[[(2~{R},3~{S},4~{R},5~{R})-5-(2-azanyl-7-methyl-6-oxidanylidene-3~{H}-purin-7-ium-9-yl)-3,4-bis(oxidanyl)oxolan-2-yl]methoxy-sulfanyl-phosphoryl] [[[(2~{R},3~{S},4~{R},5~{R})-5-(2-azanyl-7-methyl-6-oxidanylidene-3~{H}-purin-7-ium-9-yl)-3,4-bis(oxidanyl)oxolan-2-yl]methoxy-sulfanyl-phosphoryl]oxy-oxidanyl-phosphoryl] hydrogen phosphate | C22 H34 N10 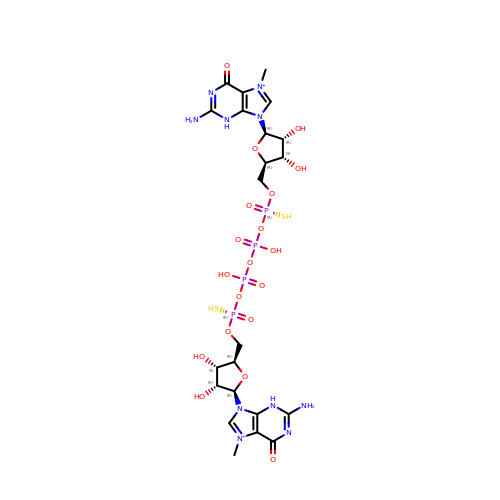O19 P4 S2 | SZQMTBAJCPCVLP-BZDQESSTSA-P>MNGKFADGPYSGILDSVLDAIGNTPMVRMKRLAKVYGLECDLLAKCEFMSAGGSVKDRIGKAMVEKAEREGRLKAGDTLIEPTSGNTGIGLALAAAVRGYRMIVTMPAKMSAEKSNIMKCLGAEIVRTPTEAAWNDENSHMGVAAKLQRELENAHILDQYNNTANPMVHYDVTAEEIITQCDGDIDMVVIGAGTGGTITGIGRKIKERCPKCKVVGVDPKGSILAVPDSLNDEKRLQSYEVEGIGYDFVPGVLDRKVVDEWVKVGDAESFTTARAIIRNEGLFVGGSSGANVWGALQAARQLKKGQKCVVLLPDSSRNYMSKFISDEWMAEHGFAPEDGAKVKEREKQFGGARIRDLLSETGATSDVPFVTARLSVEDVIKMMHETKVKEVIVTEDSEADGKTKLVGVLSE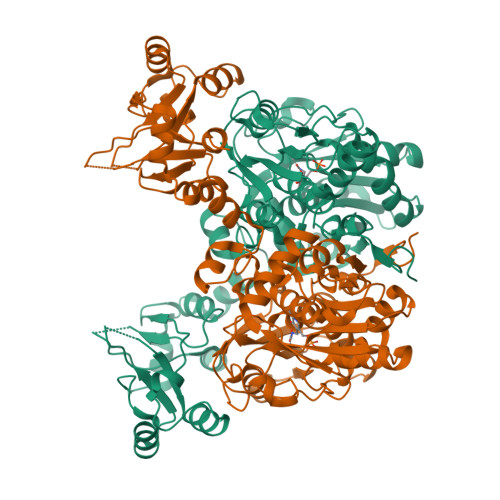DHIAHSLQSGRCAMQSPVKDIAFKKLAKALPSAYLRDVAKALDFSPYVCVMDEKPSTKKQAGMGEHERAKISLRKAGNSRECPHFLGVITRIDLLHWLATKQK[6x]A recent study demonstrated that the type V-M (formerly type V-U1, clade 2) Cas12m2 from Mycolicibacterium mucogenicum (hereafter referred to as Cas12m2 for simplicity) exhibits RNA-guided dsDNA interference activity. Cas12m2 associates with a single crRNA to recognize dsDNA targets containing a 5′-TTN-3′ PAM. Interestingly, Cas12m2 lacks target dsDNA-cleavage activity, probably due to the non-canonical His–Asp–Asp (HDD) catalytic residues in the RuvC domain, rather than the canonical, DNA-cleavable active site Asp–Glu–Asp (DED). Hence, instead of target cleavage, Cas12m2 interferes with invading MGEs through transcriptional silencing by strong DNA binding.

Most Cas12 enzymes auto-process their own pre-crRNA into mature crRNA without the involvement of a host ribonuclease. A recent study showed that, similar to Cas12a and Cas12i, Cas12m2 cleaves its pre-crRNA upstream of the crRNA scaffold, and two conserved residues (His269 and Arg270) in the WED domain may participate in crRNA maturation. His269 and Arg270 in the WED domain form base-specific interactions with the crRNA scaffold, suggesting that these residues are responsible for crRNA recognition, rather than crRNA processing. Indeed, a processing analysis of Cas12m2 revealed that alanine substitutions of His269 and Arg270 in the WED domain and Asp485 in the RuvC catalytic site had little or no effect on the pre-crRNA-processing pattern. These structural and biochemical analyses suggest that Cas12m2 may process its pre-crRNA in a unique manner. Intriguingly, when we analyzed the cryo-EM structure of Cas12m2 complexed with a 56-nucleotide crRNA, we observed an additional density close to the 5′ region of the crRNA. This density aligns well with part of the distinctive sickle-like architecture of the REC1 and REC2 domains in Cas12m2, suggesting that Cas12m2 may facilitate pre-crRNA processing through the formation of a transient asymmetric homodimer. However, because the present resolution is not sufficient to unambiguously elucidate the residues responsible for crRNA maturation, further studies are required to fully understand the pre-crRNA-processing mechanism of Cas12m2.

>[2x]MTTMTVHTMGVHYKWQIPEVLRQQLWLAHNLREDLVSLQLAYDDDLKAIWSSYPDVAQAEDTMAAAEADAVALSERVKQARIEARSKKISTELTQQLRDAKKRLKDARQARRDAIAVVKDDAAERRKARSDQLAADQKALYGQYCRDGDLYWASFNTVLDHHKTAVKRIAAQRASGKPATLRHHRFDGSGTIAVQLQRQAGAPPRTPMVLADEAGKYRNVLHIPGWTDPDVWEQMTRSQCRQSGRVTVRMRCGSTDGQPQWIDLPVQVHRWLPADADITGAELVVTRVAGIYRAKLCVTARIGDTEPVTSGPTVALHLGWRSTEEGTAVATWRSDAPLDIPFGLRTVMRVDAAGTSGIIVVPATIERRLTRTENIASSRSLALDALRDKVVGWLSDNDAPTYRDAPLEAATVKQWKSPQRFASLAHAWKDNGTEISDILWAWFSLDRKQWAQQENGRRKALGHRDDLYRQIAAVISDQAGHVLVDDTSVAELSARAMERTELPTEVQQKIDRRRDHAAPGGLRASVVAAMTRDGVPVTIVAAADFTRTHSRCGHVNPADDRYLSNPVRCDGCGAMYDQDRSFVTLMLRAATAPSNP> ADSTITIRGYVRDNR;> AKPCTVSTTNATVDLGDLYSFSLMSAGAASAWHDVALELTNCPVGTSRVTASFSGAADSTGYYKNQGTAQNIQLELQDDSGNTLN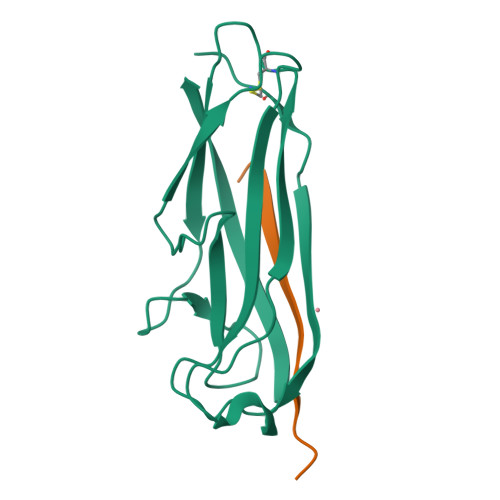TGATKTVQVDDSSQSAHFPLQVRALTVNGGATQGTIQAVISITYTYS> EVKQENRLLNESESSSQGLLGYYFSDLNFQAPMVVTSSTTGDLSIPSSELENIPSENQYFQSAIWSGFIKVKKSDEYTFATSADNHVTMWVDDQEVINKASNSNKIRLEKGRLYQIKIQYQRENPTEKGLDFKLYWTDSQNKKEVISSDNLQLPELKQKSSNSRKKRSTSAGPTVPDRDNDGIPDSLEVEGYTVDVKNKRTFLSPWISNIHEKKGLTKYKSSPEKWSTASDPYSDFEKVTGRIDKNVSPEARHPLVAAYPIVHVDMENIILSKNEDQSTQNTDSQTRTISKNTSTSRTHTSEVHGNAEVHASFFDIGGSVSAGFSNSNSSTVAIDHCLSLAGERTWAETMGLNTADTARLNANIRYVNTGTAPIYNVLPTTSLVLGKNQTLATIKAKENQLSQILAPNNYYPSKNLAPIALNAQDDFSSTPITMNYNQFLELEKTKQLRLDTDQVYGNIATYNFENGRVRVDTGSNWSEVLPQIQETTARIIFNGKDLNLVERRIAAVNPSDPLETTKPDMTLKEALKIAFGFNEPNGNLQYQGKDITEFDFNFDQQTSQNIKNQLAELNATNIYTVLDKIKLNAKMNIL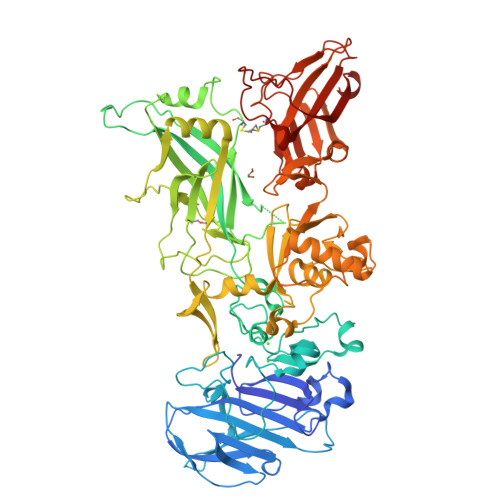IRDKRFHYDRNNIAVGADESVVKEAHREVINSSTEGLLLNIDKDIRKILSGYIVEIEDTEGLKEVINDRYDMLCISSLRQDGKTFIDFKKYNDKLPLYISNPNYKVNVYAVTKENTIINPSENGDTSTNGIKKILIFSKKGYEIG>[2x]GHELPMVERQDTD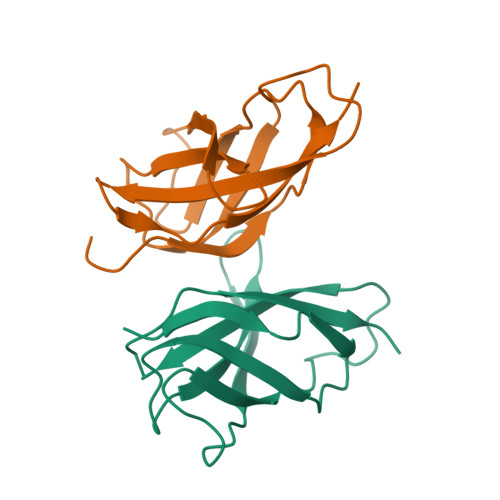SCLVYGGQQMILTGQNFTSESKVVFTEKTTDGQQIWEMEATVDKDKSQPNMLFVEIPEYRNKHIRTPVKVNFYVINGKRKRSQPQHFTYHPV>AKLVFFAEAAIIGLMV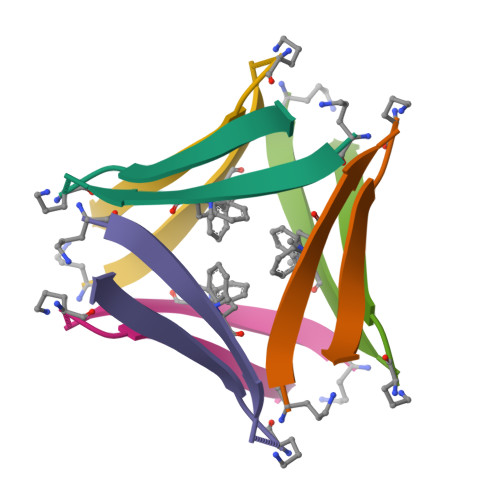[3x]>[2x]GHMASMNRTLTREQVLALAEHIENAELNVHDIGKVTNDF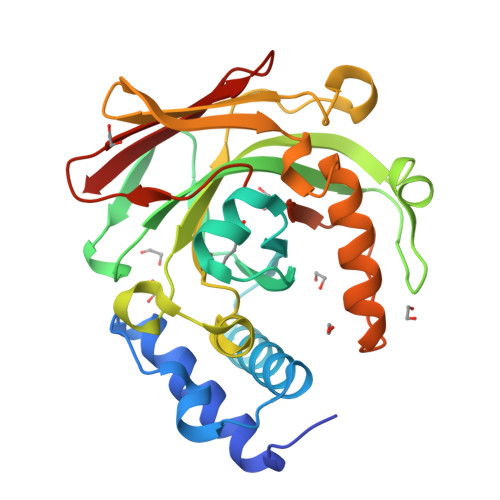PEMTFADAYDVQWEIRRRKEARGNKIVGLKMGLTSWAKMAQMGVETPIYGFLADYFSVPDGGVVDCSKLIHPKIEAEISVVTKAPLHGPGCHLGDVIAAIDYVIPTVEVIDSRYENFKFDPISVVADNASSTRFITGGRMASLEEVDLRTLGVVMEKNGEVVELGAGAAVLGHPLSSVAMLANLLAERGEHIPAGTFIMTGGITAAVPVAPGDNITVRYQGLGSVSARFI Beta-N-acetylgalactosaminidases (β-NGAs) hydrolyze the different β-GalNAc linkages of various glycans to modulate the length, combination, and abundance of glycans. Despite low sequence similarity, the crystal structures of these enzymes demonstrate that all enzymes share a prototype structure and have diversified their substrate specificities (oligosaccharide-releasing, oligosaccharide/monosaccharide-releasing, and monosaccharide-releasing) through the accumulation of mutations and insertional amino acid sequences. The overall structure of these enzymes is similar to that of CpNga123 and BvGH123, which consist of a β-sandwich domain at the N-terminus and a (β/α)8-barrel domain encompassing the catalytic region. Among Groups 1–4 and GH123, the DE motif is located at the same position, suggesting that these enzymes adopt the substrate-assisted catalysis reported for GH123 MR-β-NGAs.

In Group 4, NgaBf, NgaBl, and NgaLy were only active on GalNAc-β-pNP, highlighting their strict MR-β-NGA functionality. The structure of NgaDssm (Group 3) bore a striking resemblance to that of NgaLy and NgaP2 (Group 4) (root-mean-square distance of Cα atoms [rmsd] = 1.5–2.3 Å), while the structures of NgaLy and NgaP2 are identical (rmsd = 1.0 Å). Among the conserved amino acids, D95, W115, Y466, and R478 (amino acid numbers of NgaLy) are located at the interface between the N-terminal domain and DUF4091 (right). D95 and W115, located at the N-terminal domain, fit into the surface pocket of DUF4091, and the side chain of D95 formed hydrogen bonds with Y466 and R478 located at DUF4091. Therefore, D95, W115, Y466, and R478 are potentially important for maintaining structural integrity as they link the N-terminal and (β/α)8-barrel domains (blue letter). G427 is positioned at the entry point for the eighth β-sheet into the (β/α)8 barrel domain, with the space barely the size of the glycine residue. The DE motif (D327 and E328), Y392, and W431 are located around the substrate and are involved in substrate recognition (red letter). The Y392A and W431A mutants were purified as soluble enzymes (red letter), although their catalytic activity was considerably reduced. The Km and kcat of each enzyme for the most preferred substrate (GalNAc-β-pNP or Galβ1-3GalNAc-β-pNP) were also examined, wherein NgaLy possessed the highest kcat/Km value. Metal ions generally did not affect enzyme activity, except that of NgaLy, which was inhibited by Ni2+, Co2+, and Zn2+.

>GPGMDYQIDLVDPLTKVFADEVPDAWVVATQMVLQGEPLVLQLAYQRLRDDDASFSELTLATSLSAQCFEINQVPSQLPTWPHPDARYLRTTPGLFPDLLTPLTGPVRAYHGQVRALWLKIPTESLTPGSYELTITLTETASGQVVFSQTVPLTVAAAVAQPPRLHHTEWFSVDCLADYYHEAPYTPRLWAIIGNFMVFAHDEALMDTLLTPIFTPPLDTAVGATRTNVQLVQILPGTPYRFDWSRLRKWCQLAQQSGFAYLEMPPLFTQWGAQATPTITDTAGTALFGWHVPSTAPAYRAFLQALLPQLLAVLAEEGYDRDHLFFHLADEPNASTEDGYRAARAQVADLLDGLQVIDALSDVRFYENGLVPHPVVADDALAPFLAADAAPLWTYYCCAQTTAVPNRFFALRSYDNRVLGVLLYRHQIQGFLHWGFNFYNAQLSTRPIDPFAVTDAGGAFPSGDPFLVYPGADGQPLNSLRNEVQRLGFGDLAVLQQLEALKGRPFVERLIDVTAGMVPQFDDYPPDAGWLTRLHEKAVATLAAAAPAHKKE[4x]>[2x]SHGMAVTKVTVDGIEFPPTITPPGSSKSLTLLGAGVRGMEIETIQIKVTA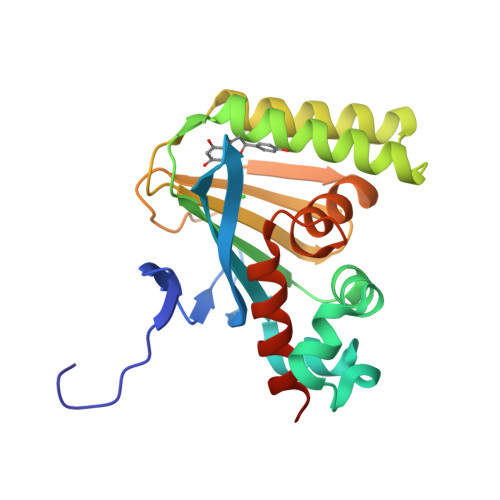IGVYAEPEVIASHLQKWKGKSASELVEDDGFFKDLVQAPVEKLVKITIIKGIKGSQYGGALEESIRDRLAALDKYSEAEEEALEEFREFFQTKSLPKGSVIFFHWPSPSTLQISVSTDGSLPEEAEATVENANVAAALLDVFLGENSVSPSTKASVAEGISALLMKNKDEKEV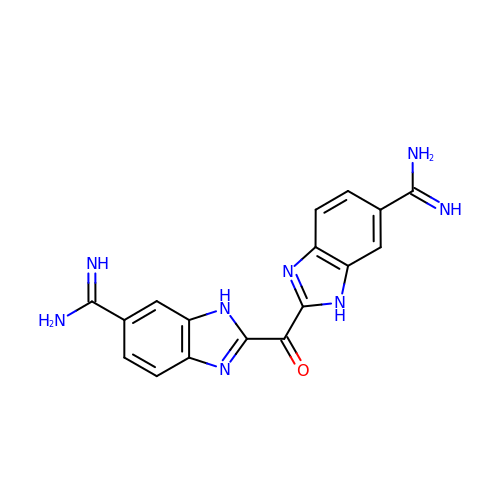BIS(5-AMIDINO-2-BENZIMIDAZOLYL)METHANONE | C17 H14 N8 O | VVVXDHROXQUONB-UHFFFAOYSA-N>MGSSHHHHHHSQDPNSSSMGQDGQQIRRDKLIIDTDPGIDDSMTILMAFRAPSVEIIGLTTIFGNVDTKGATRNALLLCERAGCPEVPVAEGSHEPLKGGKPRVADFVHGSDGIGNLFLPAPSAKKVEESAADFLINKVSEFPGEVSVLALGPLTNVALAIKRDPSF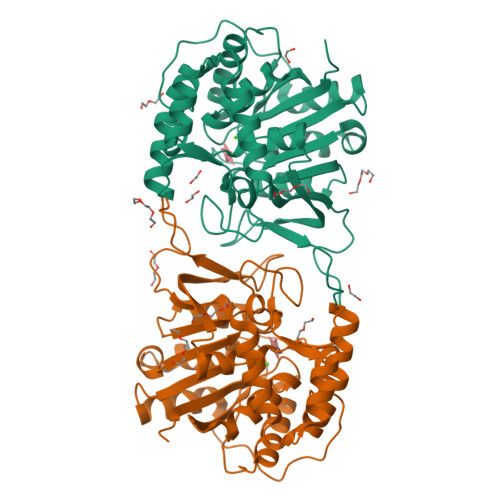ASKVKKIVVLGGAFFAAGNVNPAAEANIHGDPEAADIVFTSGADIVVVGINITTQVCLTDEDLLELRNSKGKHAAFLYEMCKFYRDWHAKSDGFHGIFLHDPVSFTAVLHPEYFTFKKGVVRVETQGICTGHTLMDQGLKKWNSENPWSGYKPISVAWTVDVPKVISFIKKLLMAP[6x]> SNAQFRQALASEHDALYNDAASPRIGAKDAKLVLVSFTDYNCPYCKRFDPLLEKITEQYPDVAVIIKPLPFKGESSAKASQAVLSVWKEDPKAFLALHQRLMQKKTMLDNASIEDAMKSTNTSKIKLTDDSLKTLQN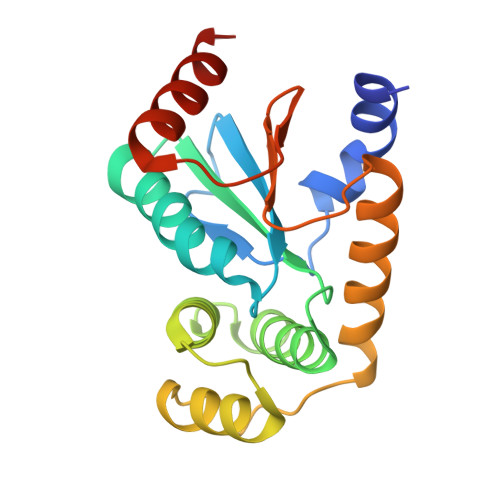NLELSRKLGIQGTPATVIGDTILPGAVDYDQLEIIVKEQLAKVKK>MASFEKAPDSVPETITGGRYSLKDGYYVYLDKQGKQVVGPKNIDNHLQYFDETTGKQVKGDFRSVNGKRIYFNANLGYADDYTTDVAGKLVGYDSNGNQVKAGYVTNSQGKTYYFNNQGEAIIGLKTDNNKTQYFGPDGAQVKGAFQQVNGKNIYFDAQTGYARQNVGFLDGTAKGFDEQGNQIKSGIATDLSGNVYYFDASGKMLTGVQNIDGKKYYFDEQGHRRRNYAGVFNNEFIYFGLDGVGQSAIEYQFEKGLTSQNSVATSHNAAKSYDTKSFTNVDGFLTANSWYRPTDILRNGTKWEPSTETDFRPLLMTWWPDKEVQANYLNYMSALGLGDQKIYTGASSQLDLNNAALIVQEAIEKKISLEKSTKWLDDSIKSFIKSKRKDIQGNLVDTNPGWTIDSETGSTNHLQNGAFIFTNSPLVPEANAAEGNRLINRTPSQQTGNHISYASQPYSGDDWGYELLLGNDVDNSNPIVQAEQLNWIHYLMNFGTITAPQDPDAHLANFDSIRIDAVDNVDADLLQIAGDYFKAAYQVGENDKNANQHIHILEDWSPNDVWYNQQVNGNSQLTMDATMQNQLLASLTRPITSRDSMKSFTKDALLVHRTADNSYNQAVPNYSFIRAHDSEVQTIIAKIISDKHPDLYPTVDKALLAKDSALYDEAFTEYNADMQKISSQKQYTHNNMPSAYAILLTNKDTVPRVYYGDLFTDNGEYMANKTPYYDAITSLLTARTKFVSGGQSLSVDKNDVLTSVRYGKGALSATDNGSSDTRNQGIGVIVSNNPNLDLNNDKVTLSMGISHAHQAYRPLLLTNSQGIVAYATDSEVPQNLYKTTNDKGELTFDASEIKGYDTVQTSGYLAVWVPVGASDEQDARTIASTEKNNGNSVYHSNAALDSQLIYEGFSNFQTVPSKNASADEYANVIIAKHAADFNKWGVTSFQMAPQYRSSTDGSFLDAVDTVQNGYAFTDRYDLGFNAADGSKNPTKYGTDEDLRNAIKSLHAQKTYDGSSIQVMADFVPDQLYNMPLEQAVSVIRTDKYGVNSENPDIQNIIYAANI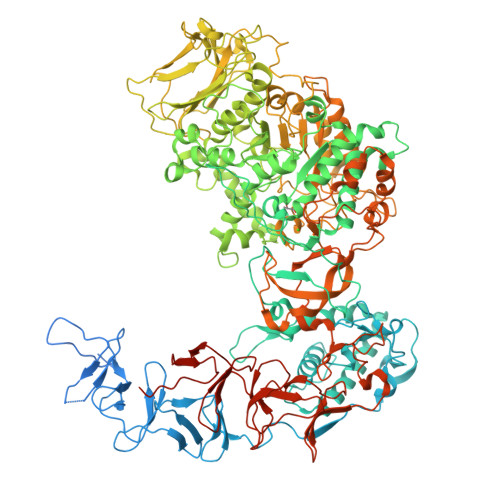KSSGTDYQSIYGGKYLAELQKNPLFKSLFDRIQISTKKTIDPNTRITQWSAKYFNGSNIQGKGINYVLKDWASNKYFNVSSNDDMYSRLPKQLMNQESNTGFIVDDIGVKYYSISGYQAKNTFVEDGNGEWYYFDNDGYMVKSTEESGPLRTVNASSKKYYILPNGVEIRNSFGQDIQGNTYYFDARGEMVTSQYISDDTQNIYYFNNDGTMAKKGGRADPAFLYKVVHHHHHH[2x]> GMNPFQNSFGGHIPQDVAGKQGENVIFIVYNLTDSPDTVDKVKDVCANFSAMIRSMRNR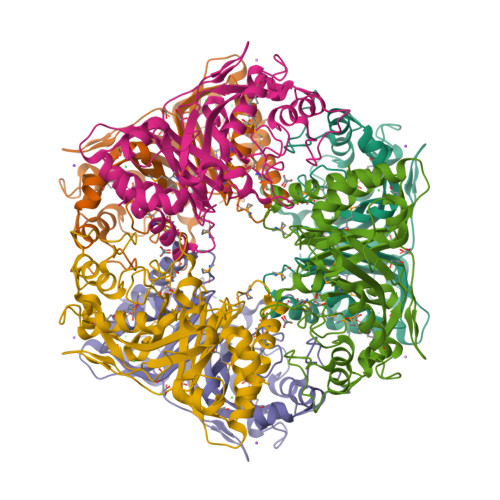FPDMQFSCTMGFGADAWTRLFPDKGKPKELSTFSEIKGEKYTAVSTPGDLLFHIRAKQMGLCFEFASILDEKLKGAVVSVDETHGFRYMDGKAIIGFVDGTENPAVDENPYHFAVIGEEDADFAGGSYVFVQKYIHDMVAWNALPVEQQEKVIGRHKFNDVELSDEEKPGNAHNAVTNIGDDLKIVRANMPFANTSKGEYGTYFIGYASTFSTTRRMLENMFIGSPAGNTDRLLDFSTAITGTLFFVPSYDLLGELGE>MNAKTKFDLYQHVTDRIIASIEAGTPAWRKPWTGEAATMQMPLRSNGEAYRGINVVMLWLTAAEKGYRSAYWFTYRQAKELGGQVRKGEKGSTVVKFGTIEREDEQTGEEKKIPYLKGYTVFNADQIDGLPEQYHAAPAEAARDLGTAADPELDAFFAATGADIRTSSEPRAYYNPTGDYIHMPPIATFHSAAGYYATLAHEATHWTGHKSRLDRFSRFSDRKSYAFEELIAEIGNCMLCASLGLIPDFDQSAAYVQSWLRALKDDKRLIFKAATEAQKAADLLQENAANFQRKEAALEHHHHHH[8x]

R388 has 35 genes assorted in functional groups or modules, among them, a gene coding for an antirestriction protein called ArdC. Interestingly, ArdC contains an N-terminal ssDNA binding domain and a C-terminal metalloprotease domain. ArdC is structurally similar to DNA-binding dependent metalloproteases involved in the maintenance of genetic stability such as Spartan or IrrE. In summary, our results indicate a new mechanism of DNA antirestriction played by protein ArdC, by which plasmids increase their conjugation host range.

The two histidines of the active site helix and the glutamic acid of the glutamate helix have been shown to coordinate a catalytic divalent metal ion, usually zinc. However, gluzinzin metalloproteases maintain the catalytic activity with Co2+, Mn2+ or Ni2+ too due to the flexibility of these three metal coordination geometries. ArdC showed increased thermal stability (assayed by ThermoFluor) in the presence of Ni2+, Mn2+ or Co2+ (ΔTM> 4°C), but not in the presence of Zn2+, Ca2+, Mg2+, Cu2+ or Fe3+. Moreover, to know the conformation of the active site when bound to metals, ArdC was crystallized in the presence of MnCl2. ArdC-Mn crystallized in the P32 space group containing eight molecules per asymmetric unit and the structure was solved at 2.7 Å. Mn2+ is tetrahedrally coordinated by H201, H205, E229 and an H2O molecule. H205 is oriented towards the metal by interaction with the conserved E228 through the non-coordinating nitrogen atom. The E202 residue of the HE202xxH motif orients and acts as a catalytic base for the activation of a water molecule that coordinates the metal. The H2O molecule could act as a Lewis acid to allow the nucleophilic attack. By analogy with other gluzinzin metalloproteases, the conserved ArdC residue Y255 could stabilize by a hydrogen bond the polypeptide chain to be cleaved.> MISDIRKDAEVRMDKCVEAFKTQISKIRTGRASPSLLDGIVVEYYGTPTPLRQLASVTVEDSRTLKINVFDRSMSPAVEKAIMASDLGLNPNSAGSDIRVPLPPLTEERRKDLTKIVRGEAEQARVAVRNVRRDANDKVKALLKDKEISEDDDRRSQDDVQKLTDAAIKKIEAALADKEAELMQF;> EYDLKRLRNIGIAAHIDAGKTTTTERILYYTGRIAVTTCFWKDHRINIIDTPGHVDFTIEVERSMRVLDGAIVVFDSSQGVEPQSETVWRQAEKYKVPRIAFANKMDKTGADLWLVIRTMQERLGARPVVMQLPIGRE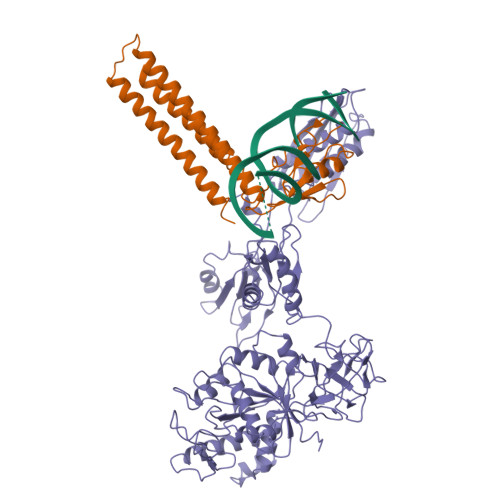DTFSGIIDVLRMKAYTYGNDLGTDIREIPIPEEYLDQAREYHEKLVEVAADFDENIMLKYLEGEEPTEEELVAAIRKGTIDLKITPVFLGSALKNKGVQLLLDAVVDYLPSPLDIPPIKGTTPEGEVVEIHPDPNGPLAALAFKIMADPYVGRLTFIRVYSGTLTSGSYVYNTTKGRKERVARLLRMHANHREEVEELKAGDLGAVVGLKETITGDTLVGEDAPRVILESIEVPEPVIDVAIEPKTKADQEKLSQALARLAEEDPTFRVSTHPETGQTIISGMGELHLEIIVDRLKREFKVDANVGKPQVAYRETITKPVDVEGKFIRQTGGRGQYGHVKIKVEPLPRGSGFEFVNAIVGGVIPKEYIPAVQKGIEEAMQSGPLIGFPVVDIKVTLYDGSYAEVDSSEMAFKIAGSMAIKEAVQKGDPVILEPIMRVEVTTPEEYMGDVIGDLNARRGQILGMEPRGNAQVIRAFVPLAEMFGYATDLRSKTQGRGSFVMFFDHYQEVPKQVQEKLI>GMTAVFRNTVLVRFKHCDAAGIVFYPRYFEMLNDFIEDWFAQALDWPFDAMHGAGQAGVPTADLHCRFVAPSRLGETLTRELRVVKL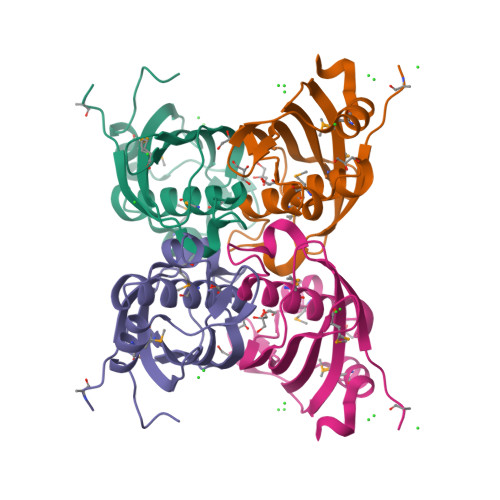GQSSFTVQVRFMGPDSGLRLEVTQRLVCVDTDKIAPRPLPDPVRQAMATYVDETLAATGSPGL[2x]>[2x]MRGSHHHHHHLVPRGSVQVISSYDQFKQVTGGDK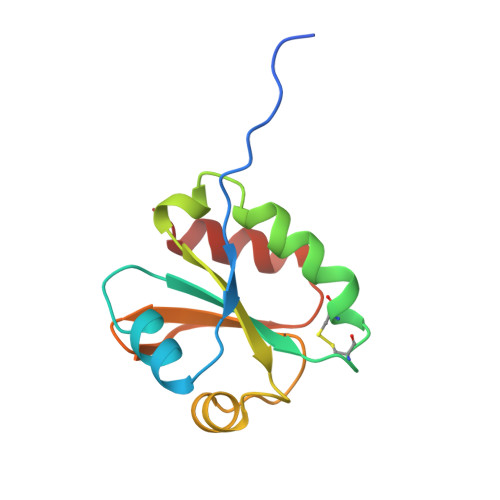VVVIDFWATWCGPCKMIGPVFEKISDTPAGDKVGFYKVDVDEQSQIAQEVGIRAMPTFVFFKNGQKIDTVVGADPSKLQAAITQHSA> GHMEDGTVRKKPKKKTQRSSEATLAPSFASLQLKKLELEFAVDPFFKKASADFDEGGAKGLLLNHLMIDSQGRIVFDSSDDAEDVAEASAKPSREADDERPDSEDADADGDISMTDRDASAPGQVETQPEEEDEDVEIDVAALGAKYFPDLSILDSLDVCPSLKTFDLGD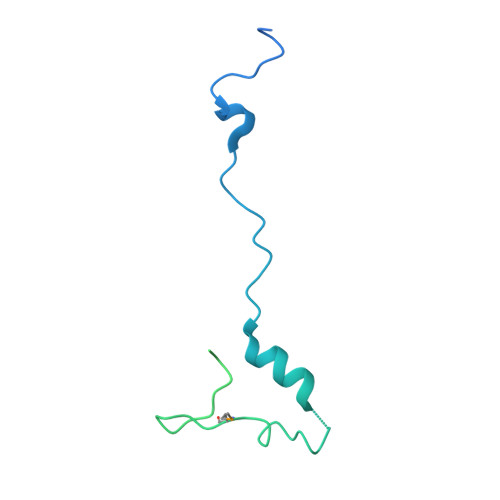PSGSLYIPFLKVPDDWRHDQEKEKTPG>GPLGSEQKKMKYLENLVGKTPMLELIFDYKGEERRIFVKNESYNLTGSIKDRMAFYTLKKAYEKNEIKKGAPIVEATSGNTGIAFSAMGAILGHPVIIYMPDWMSEERKSLIRSFGAKIILVSRKEGGFLGSIEKTKEFAKNNPDTYLPSQFSNLYNSEAHYYGIGLEIVNEMKSLNLNIDGFVAGVGTGGTVMGIGKRIKENFSNAKICPLEPLNSPTLSTGYKVAKHRIEGISDEFIPDLVKLDKLDNVVSVDD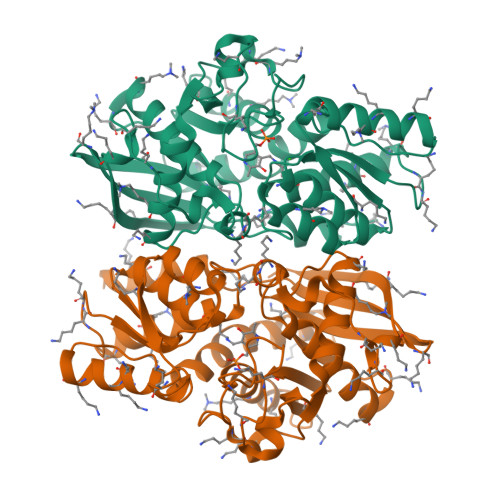GDAIVMAQKLAKCGLGVGISSGANFIGALMLQNKLGKDSVIVTVFPDDNKKYLSTDLMREEKVKEDFLSKDITLKEIKNVLRVI[4x]7-bromanyl-3~{H}-imidazo[4,5-b]pyridine | C6 H4 Br N3 | 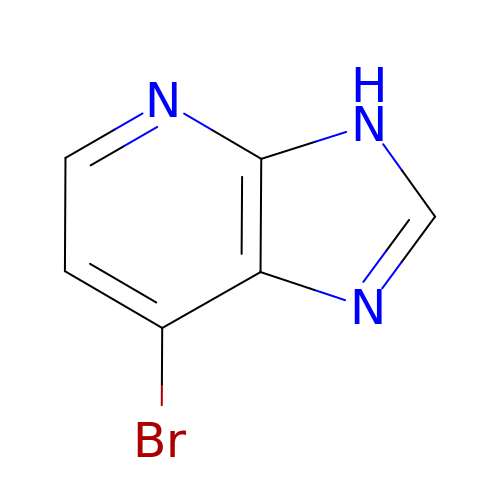DEFSPWZHYXXHLB-UHFFFAOYSA-N>MDIGINSDPPPRDWQLEKVVELSRAGIRPPTAGNREAIEAATGRPWTEWTTHDGELTGHGYAAVVNKGREEGQHYRQLGLLQAGCPTAESIYVRASPLQRTRATAQALVDGAFPGCGVAIHYANGDADPLFQTDKFAATQTDPARQLAAVKEKAGDLAQRRQALAPTIQLLKQAVCQA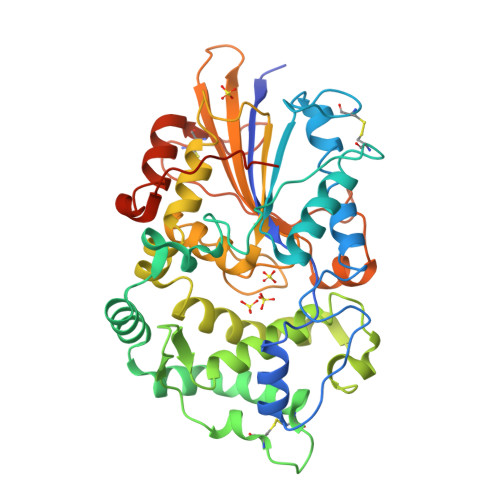DKPCPIFDTPWRVEQSKSGKTTISGLSVMANMVETLRLGWSENLPLSQLAWGKIAQASQITALLPLLTENYDLSNDVLYTAQKRGSVLLNAMLDGVKPEASPNVRWLLLVAHDTNIAMVRTLMNFSWQLPGYSRGNIPPGSSLVLERWRDAKSGERYLRVYFQAQGLDDLRRLQTPDAQHPMLRQEWRQPGCRQTDVGTLCPFQAAITALGQRIDRPSAPAVAMVLPKLAAALEHHHHHH[4x]> GGA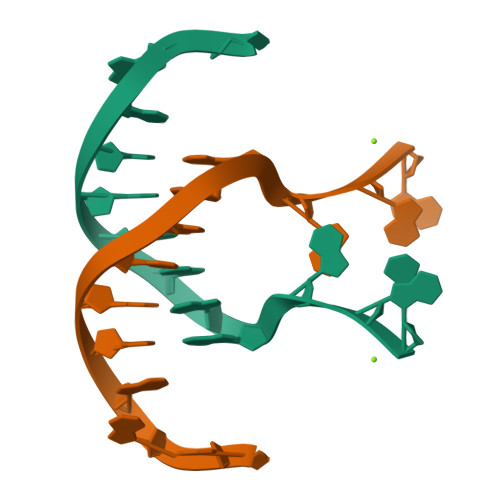AAGCTTGGAG> MLDATPKEIVERKALRINPAKTCQPVGAMYAALGIHNCLPHSHGSQGCCSYHRTVLSRHFKEPAMASTSSFTEGASVFGGGSNIKTAVKNIFSLYNPDIIAVHTTCLSETLGDDLPTYISQMED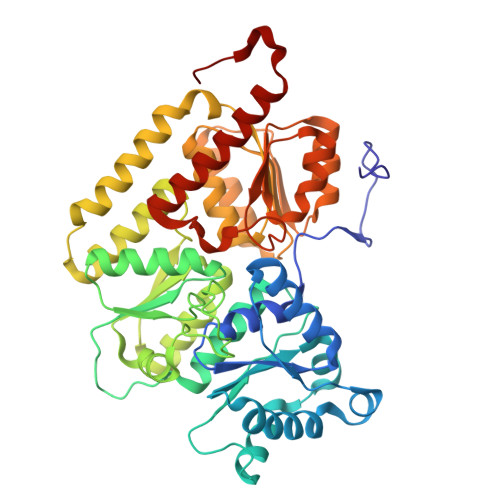AGSIPEGKLVIHTNTPSYVGSHVTGFANMVQGIVNYLSENTGAKNGKINVIPGFVGPADMREIKRLFEAMDIPYIMFPDTSGVLDGPTTGEYKMYPEGGTKIEDLKDTGNSDLTLSLGSYASDLGAKTLEKKCKVPFKTLRTPIGVSATDEFIMALSEATGKEVPASIEEERGQLIDLMIDAQQYLQGKKVALLGDPDEIIALSKFIIELGAIPKYVVTGTPGMKFQKEIDAMLAEAGIEGSKVKVEGDFFDVHQWIKNEGVDLLISNTYGKFIAREENIPFVRFGFPIMDRYGHYYNPKVGYKGAIRLVEEITNVILDKIERECTEEDFEVVR> GLSAVSKVERLMNLVIALLSTRTYLPAEKIRTTVAGYADSPSDEAFSRMFERDKNELRDLGIPLETGRVSKWDSTEGYRINRDSYALPPIGLTADEAAAVAVATQLWQSPELVTATQNAVLKLRAAGVDVDADGVGVAIASTATLPGVRGSEEVLQSLLSAIDEGRAVQFEHRPSRSADYTTRTVEPWGVVTHRGRWYLVGHDRDREDT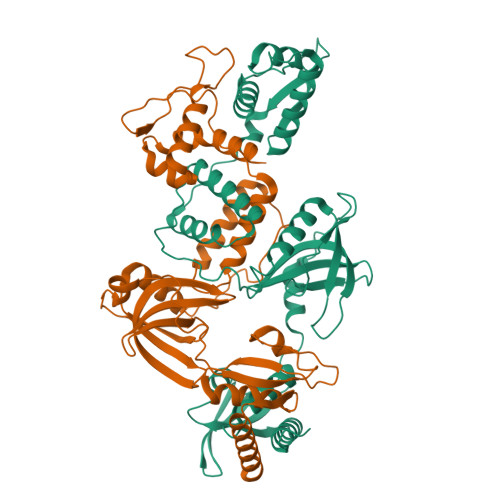RTFRLSRISAAARPIGPAGAVQKPQDVNLRDIVRRAVAEQPTGERARIWIAGGRATALRRQAVTSTPRTIGGRAGEEITVDIGTWDRLAREIASYGSDAVALEPSSLRDDVVERLRAHAAGGER;> MSQVSTRLVRLLNMVPYFQANPKVTRAEAAAALGVTGKQLDADLDQLWMCGLPGYSPGDLIDFDFVGDTIEVTFSAGVDHPLRLTSTEATGILVALRALVDVPGMVDPEAARSAIAKIESAVGSQRAVVEGITEDTSAEPGAAATVRTAVRENRALTLEYYSASRDSLATRTVDPIRVVLVGDNSYLEAWCRSAEAVRLFRFDRIVDAQLLDDPAAPPPPAVAAGPDTSLFDADPSLPSATLLIGAAAAWMFDYYPLRDITERPDGSCEATMTYASEDWMARFILGFGAEVQVLAPESLATRVRQAAEAALQAYARCV3-[(4-methoxybenzyl)amino]-6-(trifluoromethyl)quinoxaline-2-carboxylic 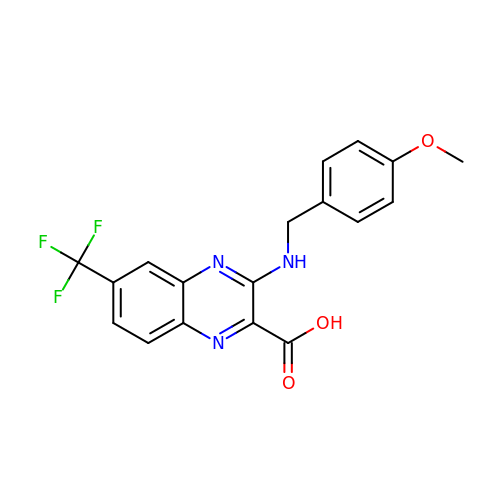acid | C18 H14 F3 N3 O3 | JWXHIZDIJHFSIP-UHFFFAOYSA-N> RGD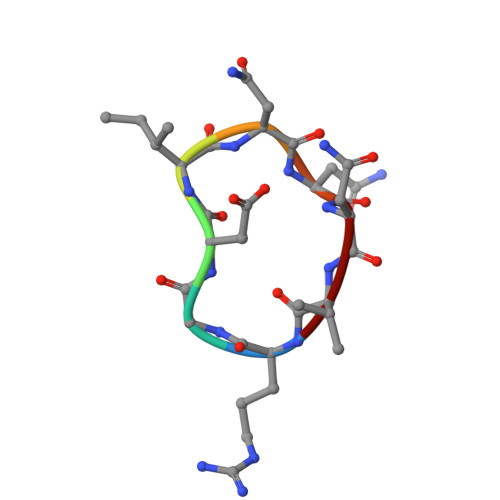INNNV>[4x]MASTKVQNPVNYITFRNEPLVKDVEKGMSQQEVLRIGGTPSGTQKRLMKPGSCNSY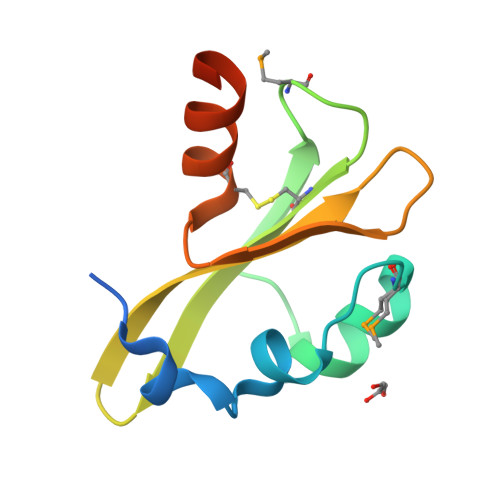ILNKDGQQQPFYVSFDGSGKVDGSGFLSCSELDRHERDARPHHHHHH> GAHMDCHLSDMLQQLHSVNASKPSERGLVRQEEAEDPACIPIFWVSKWVDYSDKYGLGYQLCDNSVGVLFNDSTRLILYNDGDSLQYIERDGTESYLTVSSHPNSLMKKITLLKYFRNYMSEHLLKAGANITPREGDELARLPYLRTWFRTRSAIILHLSNGSVQINFFQDHTKLILCPLMAAVTYI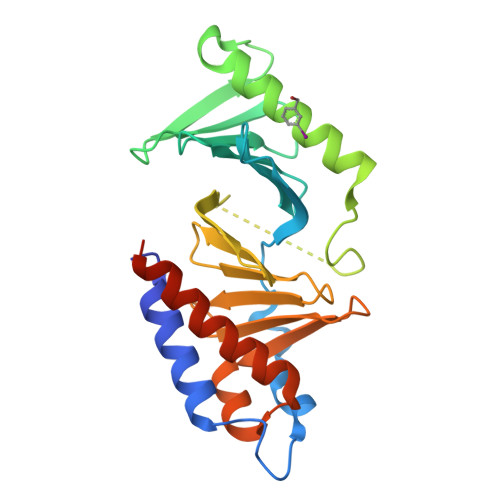DEKRDFRTYRLSLLEEYGCCKELASRLRYARTMVDKLLSSRSASNRLKAS> MTENILRKSDEEIQKEITARVKALESMLIEQGILTTSMIDRMAEIYENEVGPHLGAKVVVKAWTDPEFKKRLLADGTEACKELGIGGLQGEDMMWVENTDEVHHVVVCTLCSCYPWPVLGLPPNWFKEPQYRSRVVREPRQLLKEEFGFEVPPSKEIKVWDSSSEMRFVVLPQRPAGTDGWSEEELATLVTRESMIGVEPAKAVA;> MNGVYDVGGTDGLGPINRPADEPVFRAEWEKVAFAMFPATFRAGFRGLDEFRFGIEQMNPAEYLESPYYWHWIRTYIHHGVRTGKIDLEELERRTQYYRENPDAPLPEHEQKPELIEFVNQAVYGGLPASREVDRPPKFKEGDVVRFSTASPKGHARRARYVRGKTGTVVKHHGAYIYPDTAGNGLGECPEHLYTVRFTAQELWGPEGDPNSSVYYDCWEPYIELVDTKAAAA

Nitrile hydratase (NHase, EC 4.2.1.84), comprising α- and β-subunits, is a metalloenzyme that catalyzes nitriles into amides. The NHase active site contains either a non-heme iron or non-corrin cobalt, buried in a deep internal pocket, similar to most enzymes in nature. Hence nitrile substrates should pass through a tunnel to access the active site, and rational tunnel engineering might be a plausible choice for NHase substrate scope modification. We rationally refined the tunnel entrance region of NHase from Pseudonocardia thermophila JCM 3095 (PtNHase), based on substrate access tunnel calculations.

Two successful mutants, PtNHase-βM46R and PtNHase-βA129R, which exhibited high catalytic activity toward bulky substrates were obtained. To understand the mechanism underlying the expanded substrate scope with bulky amino acid substituents, the crystal structures of PtNHase-βM46R and PtNHase-βA129R were obtained and analyzed. Both structures had clear electron density at the mutated sites. The βArg46 and βArg129 residues were located at the “upper entrance loop” and “lower entrance loop” of the substrate access tunnel, respectively. The hydrophobic side chain of βMet46 in WT was buried and oriented towards the interior of the protein, whereas the bulky side chain of βArg46 in PtNHase-βM46R formed a hydrogen bond with a water molecule, showing an obvious outward offset to the solvent. Compared with the WT, an additional potential tunnel that started from the active site and ended at the surface entrance of the PtNHase-βM46R mutant was observed, which might provide more alternatives for bulky substrate migration. Introducing β46R and β129R mutations into PtNHase resulted in an 8.2-fold and 4.2-fold increase in activity toward pentanenitrile, and a 6.2-fold and 8.3-fold increase in activity toward cinnamonitrile, respectively. The residual activities of the WT and PtNHase-βM46R were 64.3% and 62.0%, respectively, indicating that the mutation at the βMet46 site did not significantly affect its thermostability. The maximum entrance sizes of WT, PtNHase-βM46R, and PtNHase-βA129R were estimated to be 39 Å2, 47 Å2, and 46 Å2, respectively.>[8x]MAKKTSSKGKLPPGPSPLPVLGNLLQMDRKGLLRSFLRLREKYGDVFTVYLGSRPVVVLCGTDAIREALVDQAEAFSGRGKIAVVDPIFQGYGVIFANGERWRA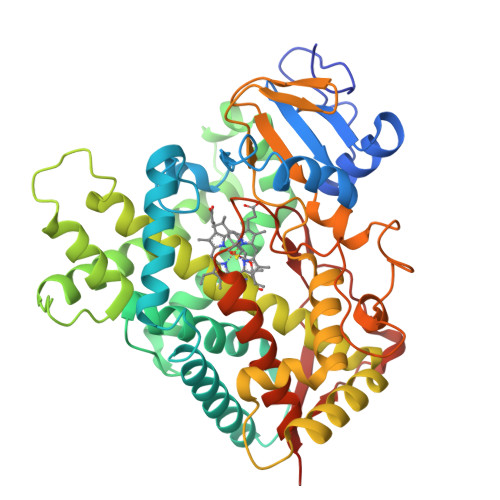LRRFSLATMRDFGMGKRSVEERIQEEARCLVEELRKSKGALLDNTLLFHSITSNIICSIVFGKRFDYKDPVFLRLLDLFFQSFSLISSFSSQVFELFSGFLKYFPGTHRQIYRNLQEINTFIGQSVEKHRATLDPSNPRDFIDVYLLRMEKDKSDPSSEFHHQNLILTVLSLFFAGTETTSTTLRYGFLLMLKYPHVTERVQKEIEQVIGSHRPPALDDRAKMPYTDAVIHEIQRLGDLIPFGVPHTVTKDTQFRGYVIPKNTEVFPVLSSALHDPRYFETPNTFNPGHFLDANGALKRNEGFMPFSLGKRICLGEGIARTELFLFFTTILQNFSIASPVPPEDIDLTPRESGVGNVPPSYQIRFLARHHHH> GGLEKDFLPLYFGWFLTKKSSETLRKAGQVFLEELGNHKAFKKELRHFISGDEPK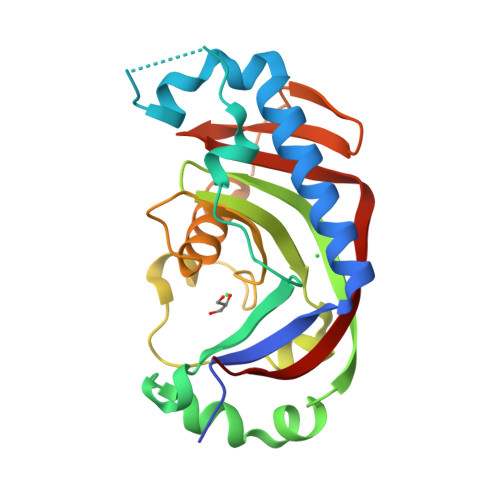EKLELVSYFGKRPPGVLHCTTKACDYGKAAGAEEYAQQEVVKRSYGKAFKLSISALFVTPKTAGAQVVLTDQELQLWPSDLDKPSASEGLPPGSRAHVTLGCAADVQPVQTGLDLLDILQQVKGGSQGEAVGELPRGKLYSLGKGRWMLSLTKKMEVKAIFTGYYG> GDVEEAIERAVVHVADTMRSGPSNSASVPALTAVETGHTSQVTPSDTMQTRHVKNYHSRSESTVENFLGRSACVYMEEYKTTDNDVNKKFVAWPINTKQMVQMRRKLEMFTYLRFDMEVTFVITSRQDPGTTLAQDMPVLT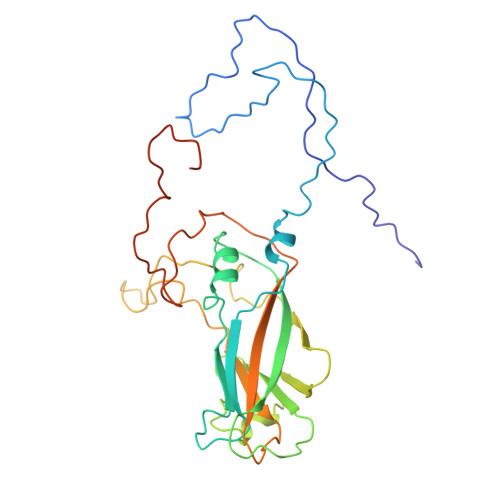HQIMYVPPGGPIPAKVDDYAWQTSTNPSIFWTEGNAPARMSIPFISIGNAYSNFYDGWSNFDQRGSYGYNTLNNLGHIYVRHVSGSSPHPITSTIRVYFKPKHTRAWVPRPPRLCQYKKAFSVDFTPTPITDTRKDINTVTTVAQSRRRGDMSTLNTH>[8x]M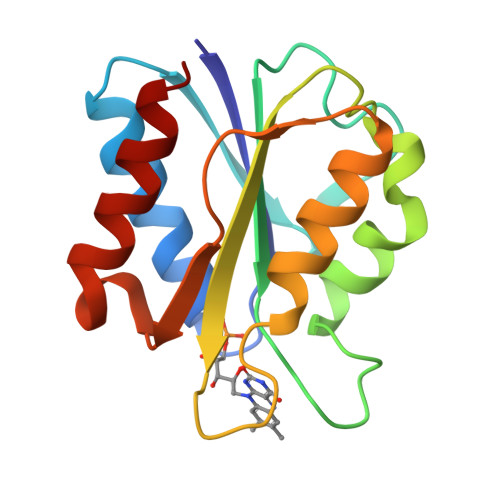SKVLIVFGSSTGNTESIAQKLEELIAAGGHEVTLLNAADASAENLADGYDAVLFGCSAWGMEDLEMQDDFLSLFEEFDRIGLAGRKVAAFASGDQEYEHFCGAVPAIEERAKELGATIIAEGLKMEGDASNDPEAVASFAEDVLKQL>MGSSHHHHHHSSGETVRFQGHMNLSQLSFHRVDQKEITQLSHLGQGTRTNVYEGRL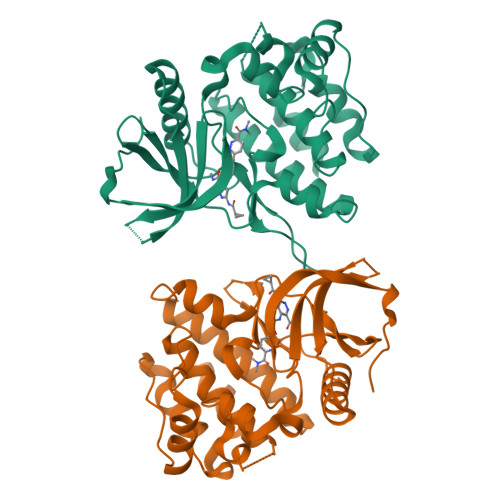RVEGSGDPEEGKMDDEDPLVPGRDRGQELRVVLKVLDPSHHDIALAFYETASLMSQVSHTHLAFVHGVCVRGPENIMVTEYVEHGPLDVWLRRERGHVPMAWKMVVAQQLASALSYLENKNLVHGNVCGRNILLARLGLAEGTSPFIKLSDPGVGLGALSREERVERIPWLAPECLPGGANSLSTAMDKWGFGATLLEICFDGEAPLQSRSPSEKEHFYQRQHRLPEPSCPQLATLTSQCLTYEPTQRPSFRTILRDLTRL[2x]>[2x]GAMVSQPIKLLVGLANPGPEYAKTRHNAGAWVVEELA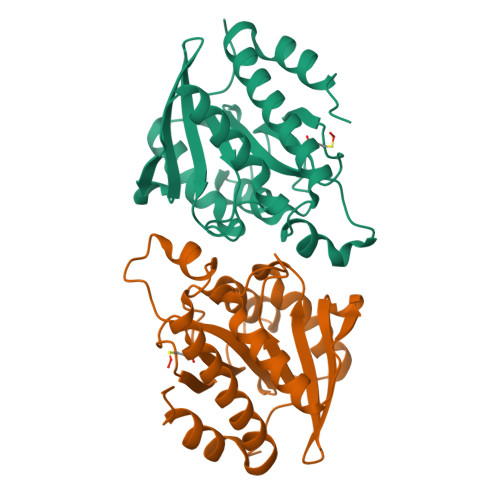RIHNVTLKNEPKFFGLTGRLLINSQELRVLIPTTFMNLSGKAIAALANFYQIKPEEIMVAHDELDLPPGVAKFKQGGGHGGHDGLKDTISKLGNNKEFYRLRLGIGHPGHKDKVAGYVLGKAPAKEQECLDAAVDESVRCLEILMKDGLTKAQNRLHTFKAE(1S,2S,3R,6R)-6-amino-4-(hydroxymethyl)cyclohex-4-ene-1,2,3-triol 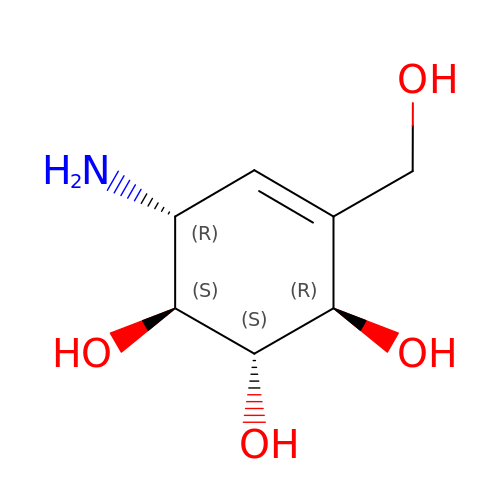| C7 H13 N O4 | XPHOBMULWMGEBA-JWXFUTCRSA-N>[6x]HHHHHHSSGLVPRGSHMASQVVRIVGVGRTGIGKLHKSVDELAASALKCALVDANMKQCDLQALIAVPSLASPQFMQAHHIATVAGLFPTKGKFIVRTVDTGGAGPITALGMAVDLVRT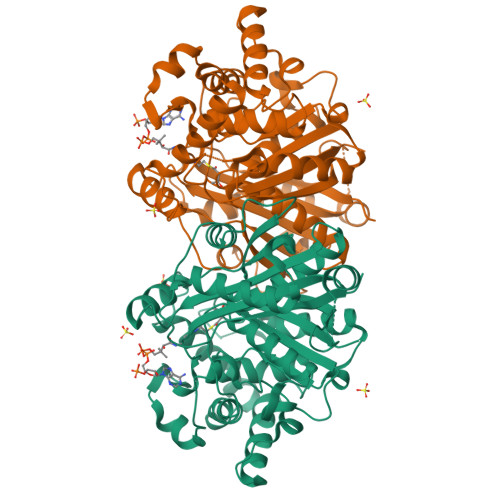RCAETVAVIAADAVLSMGSGAFAERSNASLRRSGLPEPCIPHGYDRYAQWYMSRYGLKREQLAMVPVLMSKMAERHPEAMCQKAYTLDEVLHSRCVAPVTNLLECARRADGAVALIVSGEAHYAEHFAQGKQEQRHLGGSKPIIASVAEASGPLFPPGSSDDIVPDIFSCRHAARDAFLSANLNVGDIHFFGLYDCFPICLIQAVEAVGLCPEGKGGEFMETAYNEMLNNGGVLDPSKFPINTHGGLQCFGAPWEVPAMYNITEAIAQLSEEAGDRQLTPVPKRALVYGNGGIFSASSVAILISDL> SKFLDRFRYFKQKGETFADGHGQLLNTNRDWEDGYRQRWQHDKIVRSTHGVNCTGSCSWKIYVKNGLVTWETQQTDYPRTRPDLPNHEPRGCPRGASYSWYLYSANRLKYPMMRKRLMKMWREAKALHSDPVEAWASIIEDADKAKSFKQARGRGGFVRSSWQEVNELIAASNVYTIKNYGPDRVAGFSPIPAMSMVSYASGARYLSLIGGTCLSFYDWYCDLPPASPQTWGEQTDVPESADWYNSSYIIAWGSNVPQTRTPDAHFFTEVRYKGTKTVAVTPDYAEIAKLCDLWLAPKQGTDAAMALAMGHVMLREFHLDNPSQYFTDYVRRYTDMPMLVMLEERDGYYAAGRMLRAADLVDALGQENNPEWKTVAFNTNGEMVAPNGSIGFRWGEKGKWNLEQRDGKTGEETELQLSLLGSQDEIAEVGFPYFGGDGTEHFNKVELENVLLHKLPVKRLQLADGSTALVTTVYDLTLANYGLERGLNDVNCATSYDDVKAYTPAWAEQITGVSRSQIIRIAREFADNADKTHGRSMIIVGAGLNHWYHLDMNYRGLINMLIFCGCVGQSGGGWAHYVGQEKLRPQTGWQPLAFALDWQRPARHMNSTSYFYNHSSQWRYETVTAEELLSPMADKSRYTGHLIDFNVRAERMGWLPSAPQLGTNPLTIAGEAEKAGMNPVDYTVKSLKEGSIRFAAEQPENGKNHPRNLFIWRSNLLGSSGKGHEFMLKYLLGTEHGIQGKDLGQQGGVKPEEVDWQDNGLEGKLDLVVTLDFRLSSTCLYSDIILPTATWYEKDDMNTSDMHPFIHPLSAAVDPAWEAKSDWEIYKAIAKKFSEVCVGHLGKETDIVTLPIQHDSAAELAQPLDVKDWKKGECDLIPGKTAPHIMVVERDYPATYERFTSIGPLMEKIGNGGKGIAWNTQSEMDLLRKLNYTKAEGPAKGQPMLNTAIDAAEMILTLAPETNGQVAVKAWAALSEFTGRDHTHLALNKEDEKIRFRDIQAQPRKIISSPTWSGLEDEHVSYNAGYTNVHELIPWRTLSGRQQLYQDHQWMRDFGESLLVYRPPIDTRSVKEVIGQKSNGNQEKALNFLTPHQKWGIHSTYSDNLLMLTLGRGGPVVWLSEADAKDLGIADNDWIEVFNSNGALTARAVVSQRVPAGMTMMYHAQERIVNLPGSEITQQRGGIHNSVTRITPKPTHMIGGYAHLAYGFNYYGTVGSNRDEFVVVRKMKNIDWLDGEGNDQVQESVK;> MKIRSQVGMVLNLDKCIGCHTCSVTCKNVWTSREGVEYAWFNNVETKPGQGFPTDWENQEKYKGGWIRKINGKLQPRMGNRAMLLGKIFANPHLPGIDDYYEPFDFDYQNLHTAPEGSKSQPIARPRSLITGERMAKIEKGPNWEDDLGGEFDKLAKDKNFDNIQKAMYSQFENTFMMYLPRLCEHCLNPACVATCPSGAIYKREEDGIVLIDQDKCRGWRMCITGCPYKKIYFNWKSGKSEKCIFCYPRIEAGQPTVCSETCVGRIRYLGVLLYDADAIERAASTENEKDLYQRQLDVFLDPNDPKVIEQAIKDGIPLSVIEAAQQSPVYKMAMEWKLALPLHPEYRTLPMVWYVPPLSPIQSAADAGEL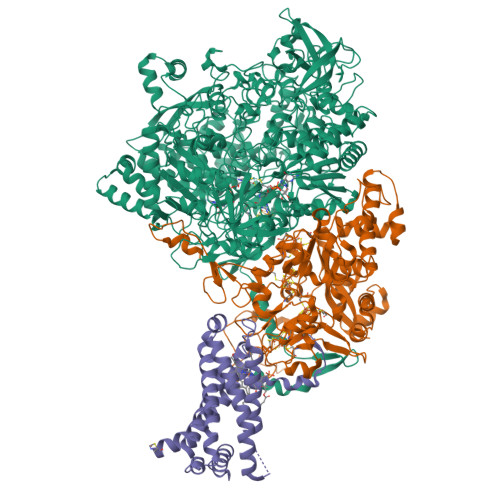GSNGILPDVESLRIPVQYLANLLTAGDTKPVLRALKRMLAMRHYKRAETVDGKVDTRALEEVGLTEAQAQEMYRYLAIANYEDRFVVPSSHRELAREAFPEKNGCGFTFGDGCHGSDTKFNLFNSRRIDAIDVTSKTEPHP;> MQFLNMFFFDIYPYIAGAVFLIGSWLRYDYGQYTWRAASSQMLDRKGMNLASNLFHIGILGIFVGYFFGMLTPHWMYEAWLPIEVKQKMAMFAGGASGVLCLIGGVLLLKRRLFSPRVRATTTGADILILSLLVIQCALGLLTIPFSAQHMDGSEMMKLVGWAQSVVTFHGGASQHLDGVAFIFRLHLVLGMTLFLLFPFSRLIHIWSVPVEYLTRKYQLVRARH>NECLGTIGPVTPLDASDFALDIRMPGVTPKESDTYFCMSMRLPVDEEAFVIDFKPRASMDTVHHMLLFGCNMPSSTGSYWFCDEGTCTDKANILYAWARNAPPTRLPKGVGFRVGGETGSKYFVLQVHYGDISAFRDNHKDCSGVSVHLTRVPQPLIAGMYLMMSVDTVIPPGEKVVNADISCQYKMYPMHVFAYRVHTHHLGKVVSGYRVRNGQWTLIGRQNPQLPQAFYPVEHPVDVTFGDILAARCVFTGEGRTEATHIGGTSS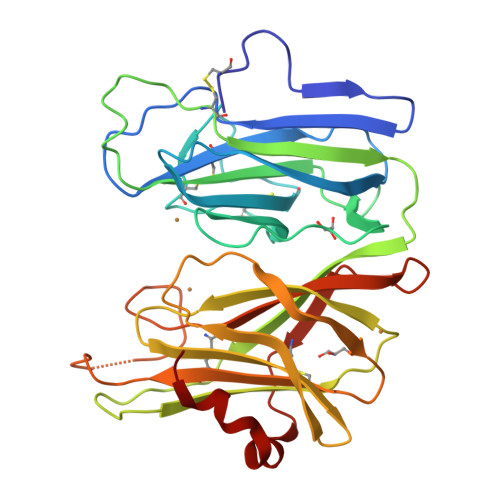DEMCNLYIMYYMEAKYALSFMTCTKNVAPDMFRTIPAEANIPI[2x]>[2x]GPLGSAMRELLLSDEYAEQKRAVNRFMLLLSTLYSLDAQAFAEAT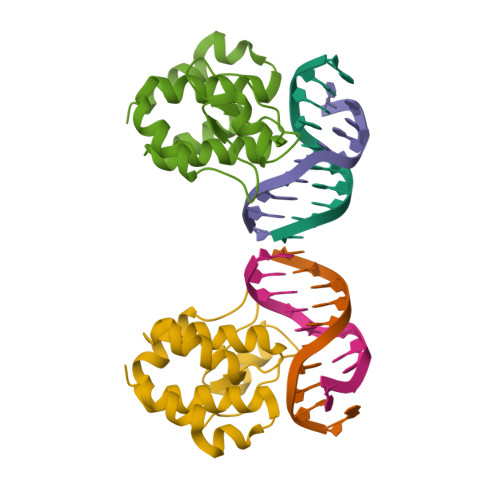ESLHGRTRVYFAADEQTLLKNGNQTKPKHVPGTPYWVITNTNTGRKCSMIEHIMQSMQFPAELIEKVCGTI5-(1~{H}-indol-3-ylmethyl)-1-methyl-~{N}-(naphthalen-1-ylmethyl)-6,7-dihydro-4~{H}-pyrazolo[4,3-c]pyridine-3-carboxamide | C28 H27 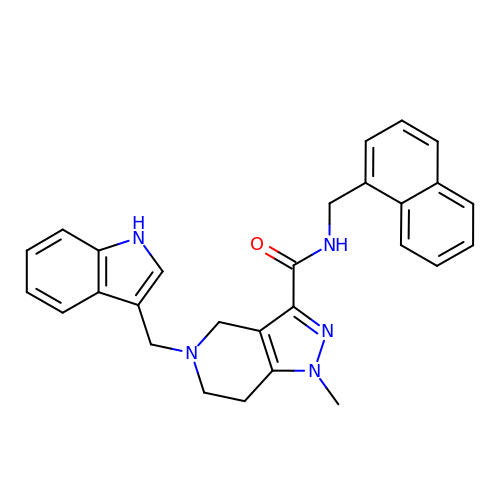N5 O | XJVZXIUKPNWOSD-UHFFFAOYSA-N The long-wavelength beamline I23 at Diamond Light Source overcomes these limitations and extends the accessible wavelength range to λ = 5.9 Å. In this study, we report the determination of diverse protein structures by experimental phasing techniques carried out at long wavelengths on beamline I23 at Diamond Light Source using S, Ca, K, Cl, V, I, Cd, and P as anomalous scatterers. Native-SAD uses light atoms naturally occurring in proteins or bound to proteins. We demonstrate that long-wavelength native-SAD has become a very compelling technique, where a low multiplicity dataset from a single crystal can be sufficient for successful structure determination, making it a general vehicle of choice for experimental phasing.

In contrast, AcrB, McjD, and A2AR diffracted to only modest resolution: 3.4, 2.8, and 2.9 Å respectively (with corresponding molecular weights of 115, 65, and 50 kDa). For McjD, two crystals were needed totaling six datasets of 360° and an overall multiplicity of 54. These examples show that S-SAD is not necessarily limited to well-diffracting crystals and the method is applicable even to more difficult membrane proteins.

>[2x]MERKQKNSLFNYIYSLMDVRGKFLFFSMLFITSLSSIIISISPLILAKITDLLSGSLSNFSYEYLVLLACLYMFCVISNKASVFLFMILQSSLRINMQKKMSLKYLRELYNENITNLSKNNAGYTTQSLNQASNDIYILVRNVSQNILSPVIQLISTIVVVLSTKDWFSAGVFFLYILVFVIFNTRLTGSLASLRKHSMDITLNSYSLLSDTVDNMIAAKKNNALRLISERYEDALTQENNAQKKYWLLSSKVLLLNSLLAVILFGSVFIYNILGVLNGVVSIGHFIMITSYIILLSTPVENIGALLSEIRQSMSSLAGFIQRHAENKATSPSIPFLNMERKLNLSIRELSFSYSDDKKILNSVSLDLFTGKMYSLTGPSGSGKSTLVKIISGYYKNYFGDIYLNDISLRNISDEDLNDAIYYLTQDDYIFMDTLRFNLRLANYDASENEIFKVLKLANLSVVNNEPVSLDTHLINRGNNYSGGQKQRISLARLFLRKPAIIIIDEATSALDYINESEILSSIRTHFPDALIINISHRINLLECSDCVYVLNEGNIVASGHFRDLMVSNEYISGLASVTE>[2x]GAHMVTSNVVLVSGEGERFTVDKKIAERSLLLKNYLNDMGDDDDEDDDEIVMPVPNVRSSVLQKVIEWAEHHRDSNFPDEDDDDSRKSAPVDSWDREFLKVDQEMLYEIILAANYLNIKPLLDAGCKVVAEMIRGRSPEEIRRTFNIVNDFTPEEEAAIR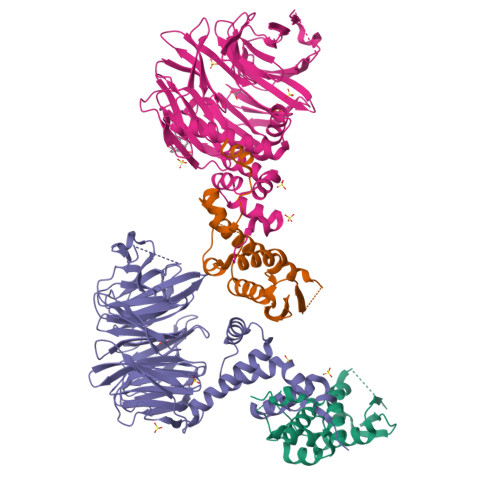RENEWAEDR;>GAGTLIKDNLKRDLITSLPFEISLKIFNYLQFEDIINSLGVSQNWNKIIRKSTSLWKKLLISENFVSPKGFNSLNLKLSQKYPKLSQQDRLRLSFLENIFILKNWYNPKFVPQRTTLRGHMTSVITCLQFEDNYVITGADDKMIRVYDSINKKFLLQLSGHDGGVWALKYAHGGILVSGSTDRTVRVWDIKKGCCTHVFEGHNSTVRCLDIVEYKNIKYIVTGSRDNTLHVWKLPKESSVPDHGEEHDYPLVFHTPEENPYFVGVLRGHMASVRTVSGHGNIVVSGSYDNTLIVWDVAQMKCLYILSGHTDRIYSTIYDHERKRCISASMDTTIRIWDLENGELMYTLQGHTALVGLLRLSDKFLVSAAADGSIRGWDANDYSRKFSYHHTNLSAITTFYVSDNILVSGSENQFNIYNLRSGKLVHANILKDADQIWSVNFKGKTLVAAVEKDGQSFLEILDFS[2x]>GPMVKPIPAEGIKSNPSKRHRDRLNTELDRLASLLPFPQDVINKLDKLSVLRLSVSYLRAKSFFDVALKSSPTERNGGQDNCRAANFREGLNLQEGEFLLQALNGFVLVVTTDALVFYASSTIQDYLGFQQSDVIHQSVYELIHTEDRAEFQRQLHWALNPSQCTESGQGIEEATGLPQTVVCYNPDQIPPENSPLMERCFICRLRCLLDNSSGFLAMNFQGKLKYLHGQKKKGKDGSILPPQLALFAIATPLQ[2x];>GPGSDAD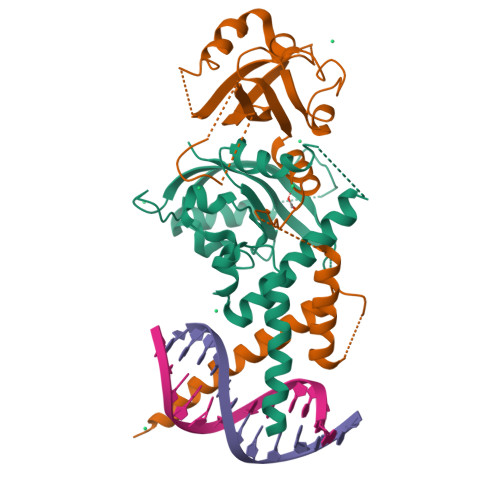KERLARENHSEIERRRRNKMTAYITELSDMVPTCSALARKPDKLTILRMAVSHMKSLRGTGNTSTDGSYKPSFLTDQELKHLILEAADGFLFIVSCETGRVVYVSDSVTPVLNQPQSEWFGSTLYDQVHPDDVDKLREQLSTSENALTGRVLDLKTGTVKKEGQQSSMRMSMGSRRSFICRMRCGTSSHFVVVHCTGYIKAWPPAGVSLPDDDPEAGQGSKFCLVAIGRLQV[2x]> MDPIHDRTSDYHKYLKVKQGDSDLFKLTVSDKRYIWYNPDPKERDSYECGEIVSETSDSFTFKTVDGQDRQVKKDDANQRNPIKFDGVEDMSELSYLNEPAVFHNLRVRYNQDLIYTYSGLFLVAVNPFKRIPIYTQEMVDIFKGRRRNEVAPHIFAISDVAYRSMLDDRQNQSLLITGESGAGKTENTKKVIQYLASVAGRNQANGSGVLEQQILQANPILEAFGNAKTTRNNNSSRFGKFIEIQFNSAGFISGASIQSYLLEKSRVVFQSETERNYHIFYQLLAGATAEEKKALHLAGPESFNYLNQSGCVDIKGVSDSEEFKITRQAMDIV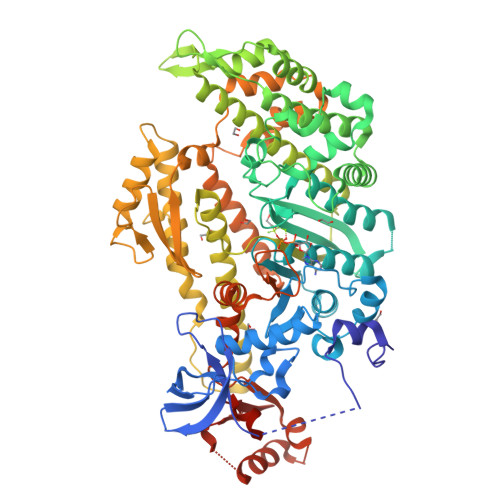GFSQEEQMSIFKIIAGILHLGNIKFEKGAGEGAVLKDKTALNAASTVFGVNPSVLEKALMEPRILAGRDLVAQHLNVEKSSSSRDALVKALYGRLFLWLVKKINNVLCEERKAYFIGVLDIEGFEIFKVNSFEQLCINYTNEKLQQFFNHHMFKLEQEEYLKEKINWTFIDFGLDSQATIDLIDGRQPPGILALLDEQSVFPNATDNTLITKLHSHFSKKNAKYEEPRFSKTEFGVTHYAGQVMYEIQDWLEKNKDPLQQDLELCFKDSSDNVVTKLFNDPNIASRAKKGANFITVAAQYKEQLASLMATLETTNPHFVRCIIPNNKQLPAKLEDKVVLDQLRCNGVLEGIRITRKGFPNRIIYADFVKRYYLLAPNVPRDAEDSQKATDAVLKHLNIDPEQFRFGITKIFFRAGQLARIEEARELRGDYKDDDDK> SKYRKKHKSEFQLLVDQARKGYK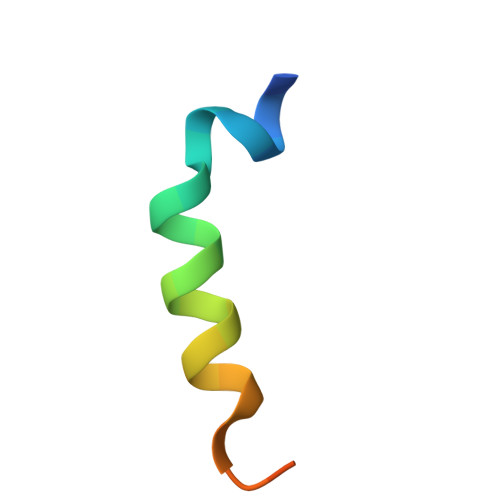KIAG>[2x]MAAHRPVEWVQAVVSRFDEQLPIKTGQQNTHTKVSTEHNKECLINISKYKFSLVISGLTTILKNVNNMRIFGEAAEKNLYLSQLIILDTLEKCLAGQPKDTMRLDETMLVKQLLPEICHFLHTCREGNQHAAELRNSASGVLFSLSCNNFNAVFSRISTRLQELTVCSEDNVDVHDIELLQYINVDCAKLKRLLKETAFKFKALKKVAQLAVINSLEKAFWNWVENYPDEFTKLYQIPQTDMAECAEKLFDLVDGFAESTKRKAAVWPLQIILLILCPEIIQDISKDVVDENNMNKKLFLDSLRKALAGHGGSRQLTESAAIACVKLCKASTYINWEDNSVIFLLVQSMVVDLKNLLFNPSKPFSRGSQPADVDLMIDCLVSCFRISPHNNQHFKICLAQNSPSTFHYVLVNSLHRIITNSALDWWPKIDAVYCHSVELRNMFGETLHKAVQGCGAHPAIRMAPSLTFKEKVTSLKFKEKPTDLETRSYKYLLLSMVKLIHADPKLLLCNPRKQGPETQGSTAELITGLVQLVPQSHMPEIAQEAMEALLVLHQLDSIDLWNPDAPVETFWEISSQMLFYICKKLTSHQMLSSTEILKWLREILICRNKFLLKNKQADRSSCHFLLFYGVGCDIPSSGNTSQMSMDHEELLRTPGASLRKGKGNSSMDSAAGCSGTPPICRQAQTKLEVALYMFLWNPDTEAVLVAMSCFRHLCEEADIRCGVDEVSVHNLLPNYNTFMEFASVSNMMSTGRAALQKRVMALLRRIEHPTAGNTEAWEDTHAKWEQATKLILNYPKAKMEDGQAAESLHKTIVKRRMSHVSGGGSIDLSDTDSLQEWINMTGFLCALGGVCLQQRSNSGLATYSPPMGPVSERKGSMISVMSSEGNADTPVSKFMDRLLSLMVCNHEKVGLQIRTNVKDLVGLELSPALYPMLFNKLKNTISKFFDSQGQVLLTDTNTQFVEQTIAIMKNLLDNHTEGSSEHLGQASIETMMLNLVRYVRVLGNMVHAIQIKTKLCQLVEVMMARRDDLSFCQEMKFRNKMVEYLTDWVMGTSNQAADDDVKCLTRDLDQASMEAVVSLLAGLPLQPEEGDGVELMEAKSQLFLKYFTLFMNLLNDCSEVEDESAQTGGRKRGMSRRLASLRHCTVLAMSNLLNANVDSGLMHSIGLGYHKDLQTRATFMEVLTKILQQGTEFDTLAETVLADRFERLVELVTMMGDQGELPIAMALANVVPCSQWDELARVLVTLFDSRHLLYQLLWNMFSKEVELADSMQTLFRGNSLASKIMTFCFKVYGATYLQKLLDPLLRIVITSSDWQHVSFEVDPTRLEPSESLEENQRNLLQMTEKFFHAIISSSSEFPPQLRSVCHCLYQVVSQRFPQNSIGAVGSAMFLRFINPAIVSPYEAGILDKKPPPRIERGLKLMSKILQSIANHVLFTKEEHMRPFNDFVKSNFDAARRFFLDIASDCPTSDAVNHSLSFISDGNVLALHRLLWNNQEKIGQYLSSNRDHKAVGRRPFDKMATLLAYLGPPEHKPVADTHWSSLNLTSSKFEEFMTRHQVHEKEEFKALKTLSIFYQAGTSKAGNPIFYYVARRFKTGQINGDLLIYHVLLTLKPYYAKPYEIVVDLTHTGPSNRFKTDFLSK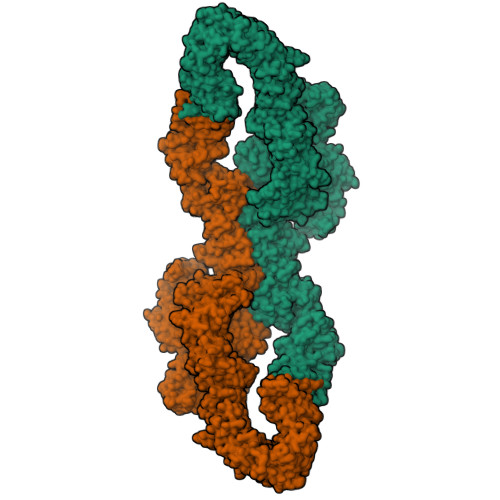WFVVFPGFAYDNVSAVYIYNCNSWVREYTKYHERLLTGLKGSKRLVFIDCPGKLAEHIEHEQQKLPAATLALEEDLKVFHNALKLAHKDTKVSIKVGSTAVQVTSAERTKVLGQSVFLNDIYYASEIEEICLVDENQFTLTIANQGTPLTFMHQECEAIVQSIIHIRTRWELSQPDSIPQHTKIRPKDVPGTLLNIALLNLGSSDPSLRSAAYNLLCALTCTFNLKIEGQLLETSGLCIPANNTLFIVSISKTLAANEPHLTLEFLEECISGFSKSSIELKHLCLEYMTPWLSNLVRFCKHNDDAKRQRVTAILDKLITMTINEKQMYPSIQAKIWGSLGQITDLLDVVLDSFIKTSATGGLGSIKAEVMADTAVALASGNVKLVSSKVIGRMCKIIDKTCLSPTPTLEQHLMWDDIAILARYMLMLSFNNSLDVAAHLPYLFHVVTFLVATGPLSLRASTHGLVINIIHSLCTCSQLHFSEETKQVLRLSLTEFSLPKFYLLFGISKVKSAAVIAFRSSYRDRSFSPGSYERETFALTSLETVTEALLEIMEACMRDIPTCKWLDQWTELAQRFAFQYNPSLQPRALVVFGCISKRVSHGQIKQIIRILSKALESCLKGPDTYNSQVLIEATVIALTKLQPLLNKDSPLHKALFWVAVAVLQLDEVNLYSAGTALLEQNLHTLDSLRIFNDKSPEEVFMAIRNPLEWHCKQMDHFVGLNFNSNFNFALVGHLLKGYRHPSPAIVARTVRILHTLLTLVNKHRNCDKFEVNTQSVAYLAALLTVSEEVRSRCSLKHRKSLLLTDISMENVPMDTYPIHHGDPSYRTLKETQPWSSPKGSEGYLAATYPTVGQTSPRARKSMSLDMGQPSQANTKKLLGTRKSFDHLISDTKAPKRQEMESGITTPPKMRRVAETDYEMETQRISSSQQHPHLRKVSVSESNVLLDEEVLTDPKIQALLLTVLATLVKYTTDEFDQRILYEYLAEASVVFPKVFPVVHNLLDSKINTLLSLCQDPNLLNPIHGIVQSVVYHEESPPQYQTSYLQSFGFNGLWRFAGPFSKQTQIPDYAELIVKFLDALIDTYLPGIDEETSEESLLTPTSPYPPALQSQLSITANLNLSNSMTSLATSQHSPGIDKENVELSPTTGHCNSGRTRHGSASQVQKQRSAGSFKRNSIKKIV>GSHMKVVYYRALYPFESRSHDEITIQPGDIVMVDESQTGEPGWLGGELKGKTGWFPANYAEKIPENEVPAPVKPVTDSTSAPAPKLALRETPAPLAVT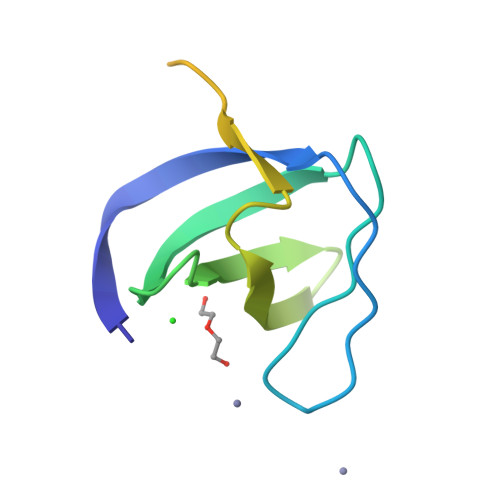S[2x]> MVPKQYPIINFTTAGATVQSYTNFIRAVRGRLTTGADVRHEIPVLPNRVGLPINQRFILVELSNHAELSVTLALDVTNAYVVGYRAGNSAYFFHPDNQEDAEAITHLFTDVQNRYTFAFGGNYDRLEQLAGNLRENIELGNGPLEEAISALYYYSTGGTQLPTLARSFIICIQMISEAARFQY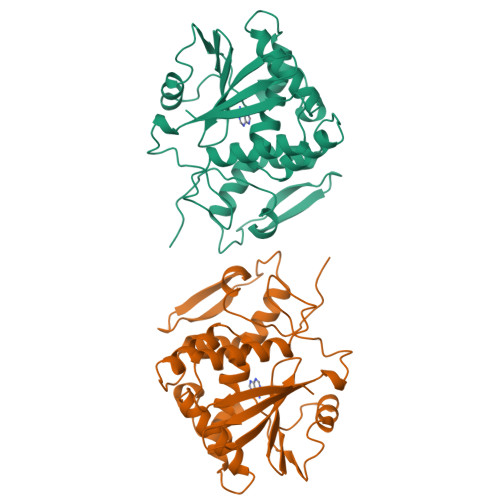IEGEMRTRIRYNRRSAPDPSVITLENSWGRLSTAIQESNQGAFASPIQLQRRNGSKFSVYDVSILIPIIALMVYRCAPPP> ERKEDIIPLANHFLKKFSRKYAKEVEGFTKSAQELLLSYPWYGNVRELKNVIER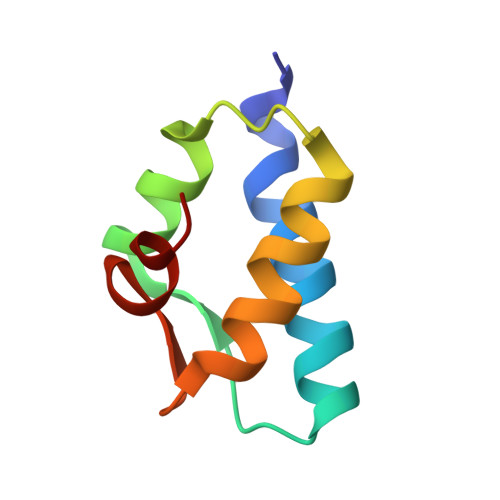AVLFSEGKFIDRGELSCLV> MLSVAARSGPFAPYLSAAAHAVPGPLXXXXXXXXXXXXXXXDLKRPLLCRESMSGRSARRDLVAGISLNAPASV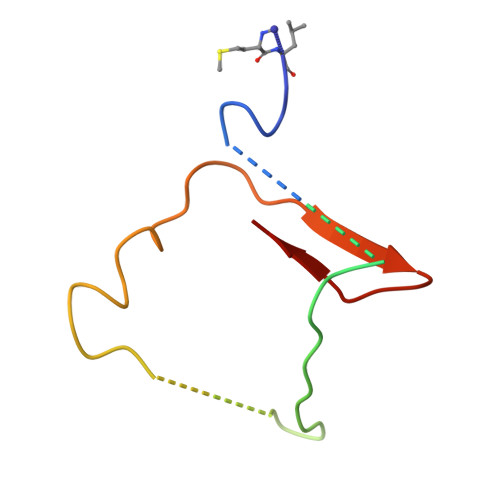RY>MADA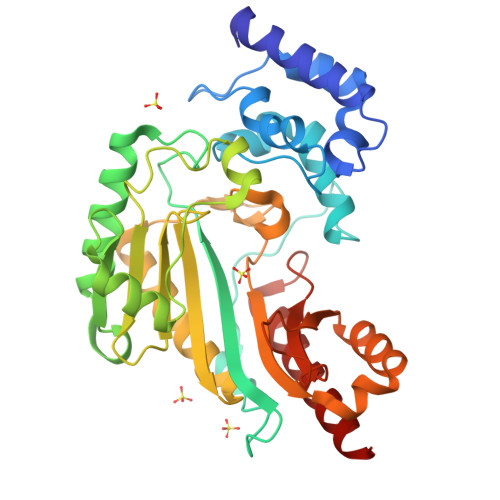ATIAKLEEGFKKLEAATDCKSLLKKYLTKSVFDQLKGKKTSLGATLLDVIQSGVENLDSGVGVYAPDAEAYTLFAPLFDPIIEDYHKGFKQTDKHPNKDFGDVNQFVNVDPDGKFVISTRVRCGRSMEGYPFNPCLTEAQYKEMESKVSSTLSNLEGELKGTYYPLTGMTKDVQQKLIDDHFLFKEGDRFLQAANACRYWPTGRGIYHNDNKTFLVWCDEEDHLRIISMQMGGDLGQVYRRLVSAVNEIEKRVPFSHHDRLGFLTFCPTNLGTTVRASVHIKLPKLAANREKLEEVAGKYSLQVRGTRGEHTEAEGGVYDISNKRRMGLTEFQAVKEMQDGILELIKIEKEMQ[2x]>[2x]HMLEMSDTMVVNGSGGVPAFLFSGSTLSSYRPNFEANSITIALPHYVDLPGRSNFKLMYIMGFPIDTEMEKDSEYSNKIRQESKISKTEGTVSYEQKITVETGQEKDGVKVYRVMVLEGTIAESIEHLDKKENEDILNNNRNRIVLADNTVINFDNISQLKEFLRRSVNIVDHDIFSSNGFEGFNPTSHFP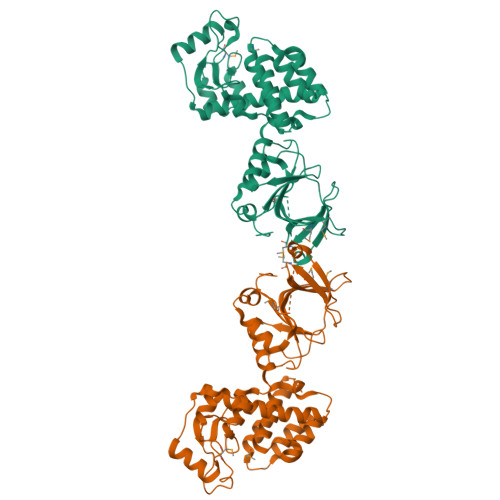SNPSSDYFNSTGVTFGSGVDLGQRSKQDLLNDGVPQYIADRLDGYYMLRGKEAYDKVRTAPLTLSDNEAHLLSNIYIDKFSHKIEGLFNDANIGLRFSDLPLRTRTALVSIGYQKGFKLSRTAPTVWNKVIAKDWNGLVNAFNNIVDGMSDRRKREGALVQKDIDSGLLK>MFVNKQFNYKDPVNGVDIAYIKIPNAGQMQPVKAFKIHNKIWVIPERDTFTNPEEGDLNPPPEAKQVPVSYYDSTYLSTDNEKDNYLKGVTKLFERIYSTDLGRMLLTSIVRGIPFWGGSTIDTELKVIDTNCINVIQPDGSYRSEELNLVIIGPSADIIQFECKSFGHDVLNLTRNGYGSTQYIRFSPDFTFGFEESLEVDTNPLLGAGKFATDPAVTLAHELIHAEHRLYGIAINPNRVFKVNTNAYYEMSGLEVSFEELRTFGGHDAKFIDSLQENEFRLYYYNKFKDVASTLNKAKSIIGTTASLQYMKNVFKEKYLLSEDTSGKFSVDKLKFDKLYKMLTEIYTEDNFVNFFKVINAKTFLNFDKA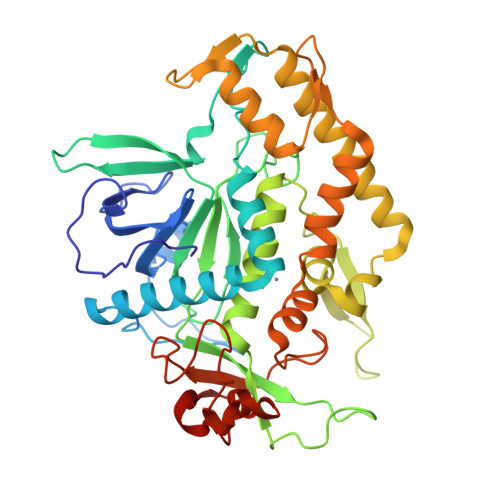VFRINIVPDENYTIKDGFNLKGANLSTNFNGQNTEINSRNFTRLKNFTGLFEFY[2x]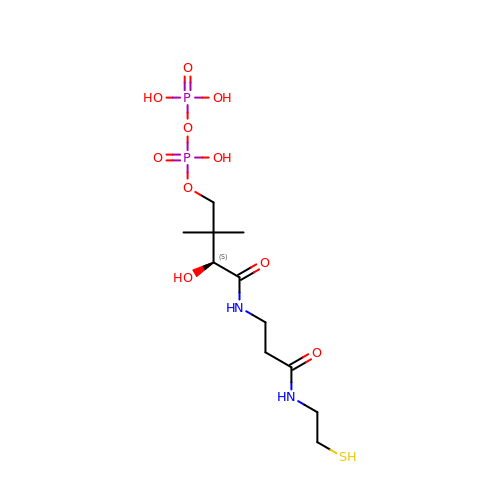[(3~{S})-2,2-dimethyl-3-oxidanyl-4-oxidanylidene-4-[[3-oxidanylidene-3-(2-sulfanylethylamino)propyl]amino]butyl] phosphono hydrogen phosphate | C11 H24 N2 O10 P2 S | UQURMDBHCKDEJS-SECBINFHSA-N P-type ATPases, including ATP7A and ATP7B, are responsible for active copper efflux that is essential for maintaining copper homeostasis in mammalian cells. These two proteins are also known as Menkes (MNK) and Wilson (WLN) disease proteins, since dysfunction of ATP7A and ATP7B leads to these diseases, respectively. ATPases contain six metal-binding domains (MBDs) that share high sequence homology with Atox1, a chaperone delivering copper to ATPase, and exhibit similar copper-binding properties. In summary, tetrathiomolybdate (TM) can react with the metal-binding domain of ATPases (WLN4) and form a Mo2S6O2-centered protein dimer.

The reaction of TM with Cu-WLN4 generated a yellow complex, and the product was purified by size-exclusion chromatography (SEC). Pale yellow crystals were obtained using the sitting-drop vapor-diffusion method. The crystal structure of the TM-WLN4 complex was determined at 1.6 Å resolution. The complex forms a protein dimer linked by a Mo2S6O2 core. Two Mo atoms are bridged by two sulfur atoms, and each protein subunit provides two thiol groups for the Mo-coordination. The Mo atom occupies the copper-binding residues (Cys14 and Cys17), preventing copper ions coordinating to this site. The Mo atom is coordinated via a pyramidal geometry, and all eight distances between Mo and S atoms (2.3−2.5 Å) are in the typical range for Mo–S covalent bonds. The two distances between Mo and O (1.5 and 1.6 Å) indicate the formation of Mo = O double bonds. Inductively coupled plasma mass spectrometry (ICP-MS) measurements showed that no copper was present in the crystal of Mo-WLN4. The absence of copper ions in the TM-WLN4 crystal structure from Cu-WLN4, together with the TM-induced dimerization of apo-WLN4, indicates that TM binding expels copper ions from the Cu-WLN4 protein.

>TCSTTLIAIAGMTCASCVHSIEGMISQLEGVQQISVSLAEGTATVLYNPAVISPEELRAAIEDMGFEASVVS[2x]> QYDDHPPVFQKKFYIGGVSEDARMFASVLRVKATDRDTGNYSAMAYRLIIPPIKEGKEGFVVETYTGLIKTAMLFHNMRRSYFKFQVIATDDYGKGLSGKADVLVSVVNQLDMQVIVSNVPPTLVEKKIEDLTEILDRYVQEQIPGAKVVVESIGARRHGDAYSLEDYSKCDLTVYAIDPQTNRAIDRNELFKFLDGKLLDINKDFQPYYGEGGRILEIRTPEAVTSIKKRGESLGYTEGASRLVPR

Hair cells have a characteristic morphology and harbor actin-filled stereocilia ‘staircases’ in which the stereocilia are coupled by protocadherin 15 (PCDH15) molecules from one stereocilium linked with cadherin 23 (CDH23) molecules from an adjacent stereocilium. Upon movement of the stereocilia induced by fluctuations of the surrounding fluid, the PCDH15-CDH23 ‘tip links’ trigger the opening of a mechano-electrical transduction (MET) ion channel at the stereocilia tips. PCDH15 belongs to the cadherin superfamily and consists of 11 extracellular cadherin (EC) domains, an extracellular linker (EL) domain, a single transmembrane (TM) helix and a cytoplasmic domain. Here we demonstrate that PCDH15 forms a robust complex with LHFPL5 and that the assembly is composed of 2 copies of each protein, thus providing concrete evidence that the composition of PCDH15 in the tip link is a dimer.

We therefore expressed the EC11-EL construct as a secreted protein from mammalian cells and solved the structure at a resolution of ~1.4 Å by x-ray crystallography. As expected, the EC11 domain shows a classic cadherin fold, while the EL domain has a ferredoxin-like fold. The EC11-EL construct forms a 2-fold symmetric dimer in the crystal lattice. Unlike the linear ‘top to bottom’ arrangement of cadherin domains, the EC11 and EL domains sit ‘side-by-side’, providing extensive interactions within each protomer and throughout the dimer interface. A ‘major’ dimer interface is formed by contacts between EC11 and the EL domain of the symmetry related protomer (EL’). A ‘minor’ dimer interface is defined by contacts between EC11 on one protomer and EC11 on the second protomer (EC11’). A top-down view of the EC11-EL dimer illustrates how residues from α1b and α2b of EL form a negatively charged cavity harboring a deafness mutation, Q1347K, at the end of the α2b helix. We also note that there is a strong density in the x-ray maps with a ring-like feature located next to Ser1167, suggestive of O-linked glycosylation. We examined the fit of galactose, mannose and glucose to the density and found that mannose fit best. Although the mannose moiety does not directly interact with other residues, it fills the EC11-EL dimer cavity and may help stabilize the dimer.[3,4-bis(oxidanyl)phenyl]-phenyl-methanone | 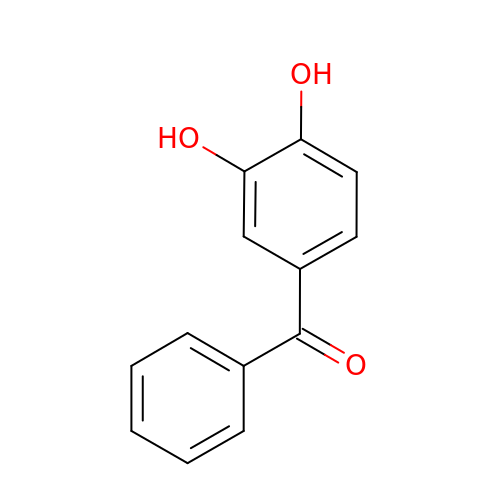C13 H10 O3 | ARWCZKJISXFBGI-UHFFFAOYSA-N>[4x]MINPVTNTQGVSPINTKYAEHVVKNIYPEIKHDYFNESPNIYDKKY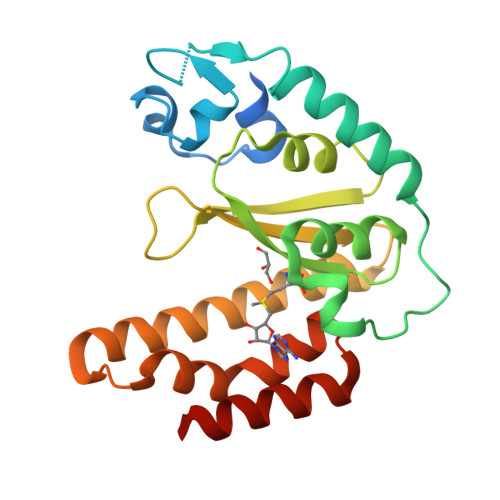ISGITRGVAELKQEEFVNEKARRFSYMKTMYSVCPEAFEPISRNEASTPEGSWLTVISGKRPMGQFSVDSLYNPDLHALCELPDICCKIFPKENNDFLYIVVVYRNDSPLGEQRANRFIELYNIKRDIMQELNYALPELKAVKSEMIIAREMGEIFSYMPGEIDSYMKYINNKLSKIE N-[7-KETO-8-AMINOPELARGONIC 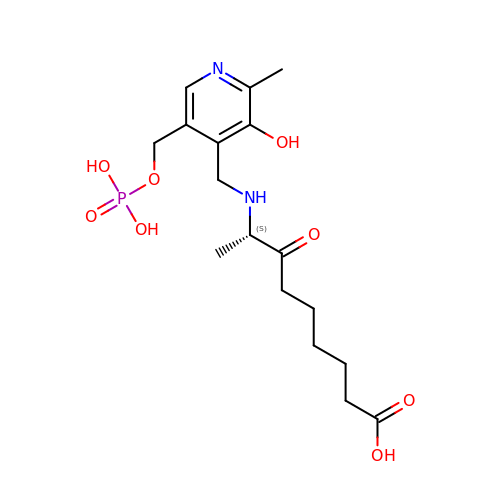ACID]-[3-HYDROXY-2-METHYL-5-PHOSPHONOOXYMETHYL-PYRIDIN-4-YL-METHANE] | C17 H27 N2 O8 P | YXEXNGWPUWJMIT-NSHDSACASA-N>VSFRQKRTRIPLLAMTVTALAAAVCGVTTAPAATGAEVAVPLSVGAAAGNATPIPGYVIQSSAQVSDDSAVSKPGFPTSGWYPVSSRSTVYAGLLQNGKYADPFYSTNMQNVPAAQFSVPWWYRTDLNVDDTSSRTYLDFSGVLSKADVWVNGTKVATKDQVNGAYTRHDLDITAQVHTGVNSVAFKVYPNDPNRDLSMGWIDWAQTPPDQNMGIVRDVLVRRSGAVALRSAHVIQKLNSALDHADLTVKADVRNDSANAVQTTVAGTVAGKPISQTVSLAAKERKTVTFPLVGLDRPNVWWPAGMGGQHRYDLDLTASVGGTPSDAAKSKFGVRDVKATLNSSGGRQYSVNGKPLLIRGGGYTPDLFLRWNETAAADKLKYVLNLGLNTVRLEGHIEPDEFFDIADDLGVLTMPGWECCDKWEGQVNGEEKGEPWVESDYPIAKASMFSEAERLRDHPSVISFHIGSDFAPDRRIEQGYLDAMKAADFLLPVIPAASARPSPITGASGMKMNGPYDYVPPVYWYDKSQKDRGGAWSFNSETSAGVDIPTMDTLKRMMSASELDTMWKNPSAKQYHRSSSDTFGNLKLFGDALTKRYGASANLNDFVRKAQLSQYENVRAEFESHSRNYTDSTNPSTGLIYWMLNSPWTSLHWQLFDAYMDQNGAYYGAKKANEPLHIQYSHDNRSVVVINQTSNAVSGLTATTKLYNLDGTEKYSNTKTGLSVGALGAKATAVTVPAVSGLSTTYLAKNVLTDSSGKEVSRNVYWLSTKADTLNWGGSDWY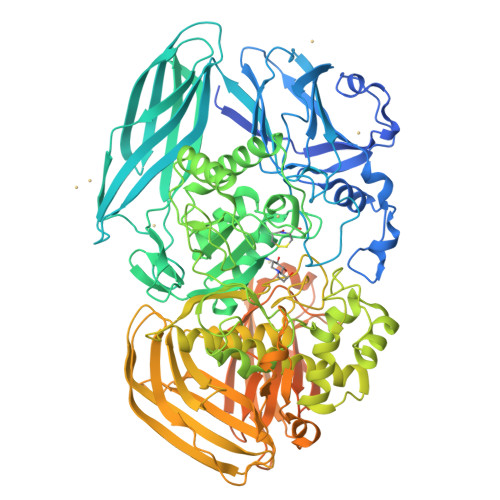YTPQSAFADLSGLNNLGQSAVGATANSVAGADGTTTTTVTLKNTSGGRLPAFYVDSKVVDSAGKPVLPVEWNDNAVSLWPGETTTLTAKYRTADLKGSKPSVRISGWNTGTQTVPADGSGPGPSDPVDYQAEDATIVQGAVESNHAGYTGTGFVNYDNVAGSSVEWTVTVPSAGTYDVVVRYANGTTTSRPLDFSVNGSISASGVAFGSTGTWPAWTTKTVRVTLAAGVNKIKAVATTANGGPNVDKITL[2x]> GEEELQENQELIREKS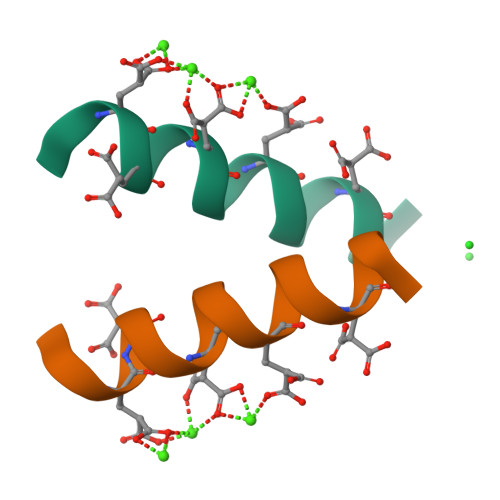NX2-hydroxy-5-methylbenzoic acid | C8 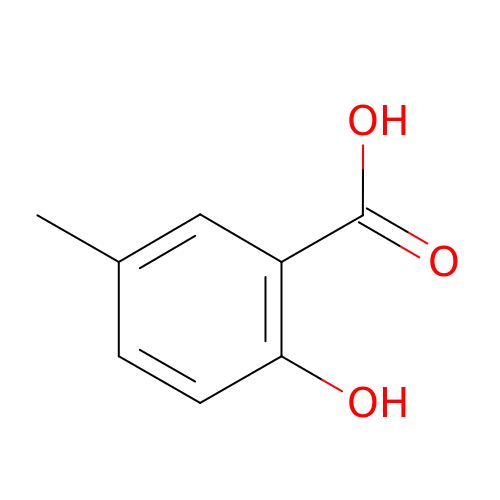H8 O3 | DLGBEGBHXSAQOC-UHFFFAOYSA-N>MLNRVVLVGRLTKDPEYRTTPSGVSVATFTLAVNRTFTNAQGEREADFINCVVFRRQADNVNNYLSKGSLAGVDGRLQSRNYENQEGRRVFVTEVVCDSVQFLEPHHHHHH[2x]

Single-stranded DNA-binding proteins (SSBs) play a crucial role in DNA metabolism by binding and stabilizing single-stranded DNA (ssDNA) intermediates. The majority of SSBs adopt homotetrameric configurations for activity. Diverging from E. coli, which harbors a solitary SSB variant (EcSSB), certain bacteria like Staphylococcus aureus exhibit a more complex scenario with the presence of three paralogous SSBs, specifically referred to as SaSsbA, SaSsbB, and SaSsbC. Of these, SaSsbA may be an EcSSB counterpart due to its possession of an acidic tip and sequence resemblance to EcSSBn.

For the investigation of the binding mode, we solved the complexed crystal structure of SaSsbA with 5-FU at a resolution of 2.3 Å. The individual monomer within this complexed SaSsbA revealed the characteristic OB-fold structure, featuring a β-barrel comprising 5 β-strands capped with an α-helix. Within this complex structure of a SaSsbA dimer, a single glycerol molecule and one 5-FU molecule were encapsulated. The positioning of this glycerol molecule, designated as Glycerol 3, within the SaSsbA–5-FU complex closely mirrored that of Glycerol 1 within the glycerol-bound SaSsbA. Residues R18, P21, V52, F54, Q78, R80, E94, and V96, positioned within a contact distance of <4 Å, were instrumental in the binding of 5-FU. Based on interactions discerned via PLIP, the four side chains of R18, Q78, R80, and E94 were observed to form hydrogen bonds with 5-FU. The electrostatic potential surface of the SaSsbA complexed with 5-FU unveiled that 5-FU effectively occupied the groove within SaSsbA, a site significant for single-stranded DNA binding. The positive (blue) and negative (red) charge distributions underscored that several critical basic residues on the SaSsbA surface, which are exposed to the solvent and collectively form a binding pathway conducive for accommodating ssDNA binding ssDNA (gold). This complex structure insightfully revealed that the presence of 5-FU in the groove potentially influences the wrapping of ssDNA by SaSsbA. Notably, a substantial conformational change was observed in R18 upon 5-FU binding, resulting in a shift of its side chain position by 7.2 Å and an angular alteration of 77.4°. However, intriguingly, our complexed structure revealed distinct 5-FU binding configurations for SaSsbA and SaSsbB.> MKDLLKFLKAQTKTEEFDAIKIALASPDMIRSWSFGEVKKPETINYRTFKPERDGLFCARIFGPVKDYECLCGKYKRLKHRGVICEKCGVEVTQTKVRRERMGHIELASPTAHIWFLKSLPSRIGLLLDMPLRDIERVLYFESYVVIEGGMTNLERQQILTEEQYLDALEEFGDEFDAKMGAEAIQALLKSMDLEQECEQLREELNETNSETKRKKLTKRIKLLEAFVQSGNKPEWMILTVLPVLPPDLRPLVPLDGGRFATSDLNDLYRRVINRNNRLKRLLDLAAPDIIVRNEKRMLQEAVDALLDNGRRGRAITGSNKRPLKSLADMIKGKQGRFRQNLLGKRVDYSGRSVITVGPYLRLHQCGLPKKMALELFKPFIYGKLELRGLATTIKAAKKMVEREEAVVWDILDEVIREHPVLLNRAPTLHRLGIQAFEPVLIEGKAIQLHPLVCAAYNADFDGDQMAVHVPLTLEAQLEARALMMSTNNILSPANGEPIIVPSQDVVLGLYYMTRDCVNAKGEGMVLTGPKEAERLYRSGLASLHARVKVRITEYEKDANGELVAKTSLKDTTVGRAILWMIVPKGLPYSIVNQALGKKAISKMLNTCYRILGLKPTVIFADQIMYTGFAYAARSGASVGIDDMVIPEKKHEIISEAEAEVAEIQEQFQSGLVTAGERYNKVIDIWAAANDRVSKAMMDNLQTETVINRDGQEEKQVSFNSIYMMADSGARGSAAQIRQLAGMRGLMAKPDGSIIETPITANFREGLNVLQYFISTHGARKGLADTALKTANSGYLTRRLVDVAQDLVVTEDDCGTHEGIMMTPVIEGGDVKEPLRDRVLGRVTAEDVLKPGTADILVPRNTLLHEQWCDLLEENSVDAVKVRSVVSCDTDFGVCAHCYGRDLARGHIINKGEAIGVIAAQSIGEPGTQLTMRTFHIGGAASRAAAESSIQVKNKGSIKLSNVKSVVNSSGKLVITSRNTELKLIDEFGRTKESYKVPYGAVLAKGDGEQVAGGETVANWDPHTMPVITEVSGFVRFTDMIDGQTITRQTDELTGLSSLVVLDSAERTAGGKDLRPALKIVDAQGNDVLIPGTDMPAQYFLPGKAIVQLEDGVQISSGDTLARIPQESGGTKDITGGLPRVADLFEARRPKEPAILAEISGIVSFGKETKGKRRLVITPVDGSDPYEEMIPKWRQLNVFEGERVERGDVISDGPEAPHDILRLRGVHAVTRYIVNEVQDVYRLQGVKIND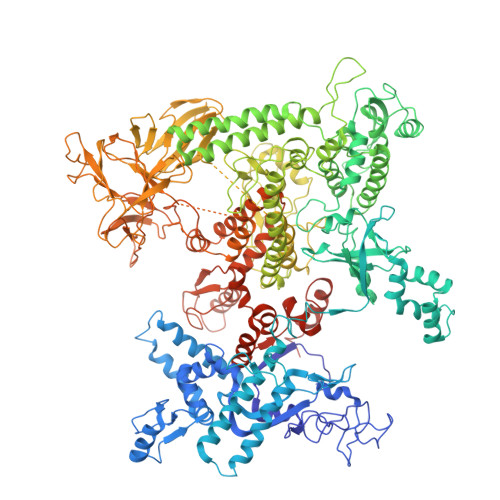KHIEVIVRQMLRKATIVNAGSSDFLEGEQVEYSRVKIANRELEANGKVGATYSRDLLGITKASLATESFISAASFQETTRVLTEAAVAGKRDELRGLKENVIVGRLIPAGTGYAYHQDRMRRRAAGEAPAAPQVTAEDASASLAELLNAGLGGSDNELEVHHHHHH>[2x]DAEKLAASSLFTWDFDALDKSDEDLTAVCVRVFQELHVIEQFNIDEKKLRKWLQKVRTQYNKNPFHNWRHAVMVLHTTYLLLTSVATEFITEVELLAMLIAALS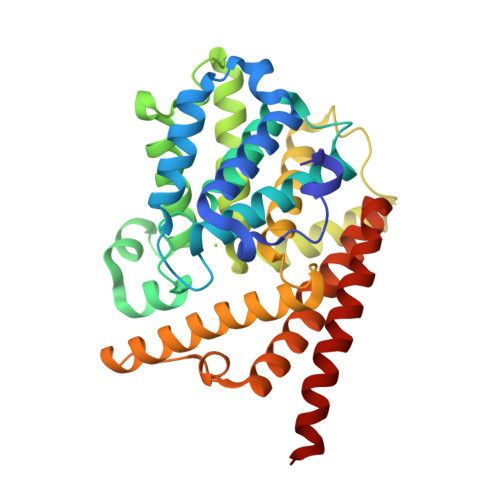HDLDHNGLTNAFHINSRSELALVYNDQSVLENHHSHLAFEILLEKGCNVVENLDEDEFKRLRAVIINCILNTDMATHHTKLSKMEEVNRLGGFINLAENNDQRLFVLAVLLHTADLHNPIKPFESNKRWSARLQKEFNNQVELEAKMNLPSLPFMRGNDEESLAKGEIGFINFVVKPWHQQLSQAFPKLDFLLDTIDANLAEWKAIAESYRQMH>[2x]I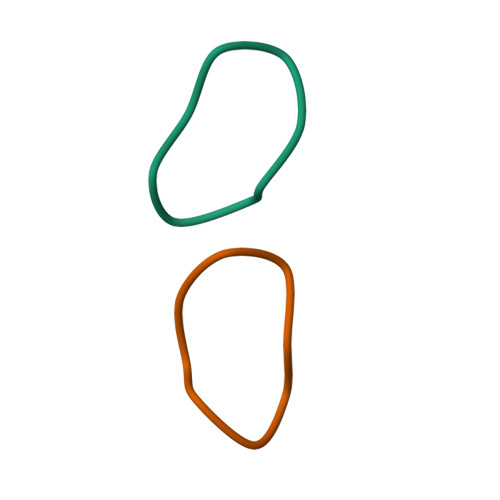LGSIILG> DEASGIGPEEHFPEVPEIEPMGPVCPFRCQCHLRVVQCSDLGLEKVPKDLPPDTALLDLQNNKITEIKDGDFKNLKNLHTLILINNKISKISPGAFAPLVKLERLYLSKNQLKELPEKMPKTLQELRVHENEITKVRKSVFNGLNQMIVVELGTNPLKSSGIENGAFQGMKKLSYIRIADTNITTIPQGLPPSLTELHLDGNKITKVDA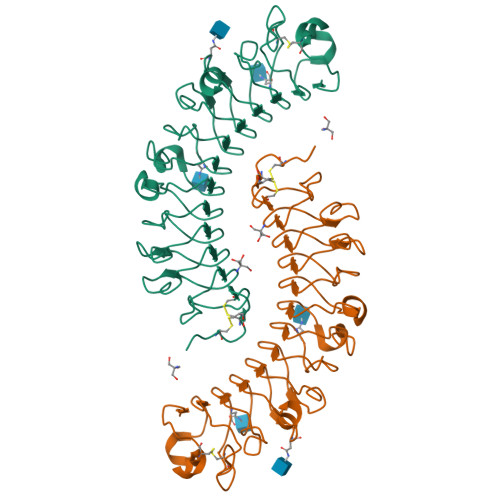ASLKGLNNLAKLGLSFNSISAVDNGSLANTPHLRELHLNNNKLVKVPGGLADHKYIQVVYLHNNNISAIGSNDFCPPGYNTKKASYSGVSLFSNPVQYWEIQPSTFRCVYVRAAVQLGNY> PKNLNLWGKYLRLVGRGARRGFKKWQVIPPIPVKAYGREPSAASQTGLYHDEDFNYHTKRTFSMRRTRRKIKPNVFRRTFTSSLLNVTIPNVRVTTSALHAMDDMGGFDAYILRTPPQELRSHMGERMRQVMYYYQDQPAIRDWGLPWKVFLKVASRRDPFYACYRHNLRKQQYEADLR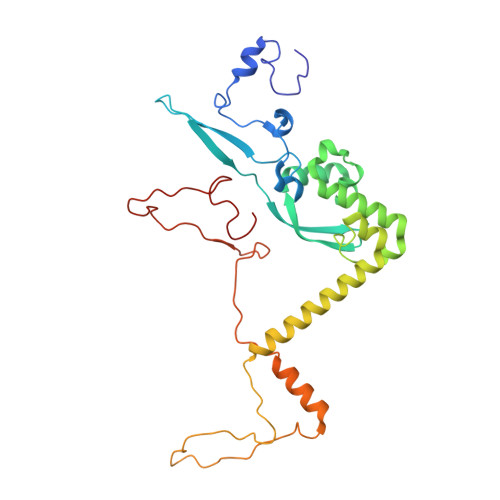SRVRSFSPYYLPSGHQPHAERQVFHEGAGESPPLNLWWRENRELEEAFRRRLGEAKCFERAFADSSEPLGYTKGRCRGGGGKSGRSVRRRSKTHKYRENRAF>GGCUCGGCGGCGGA[2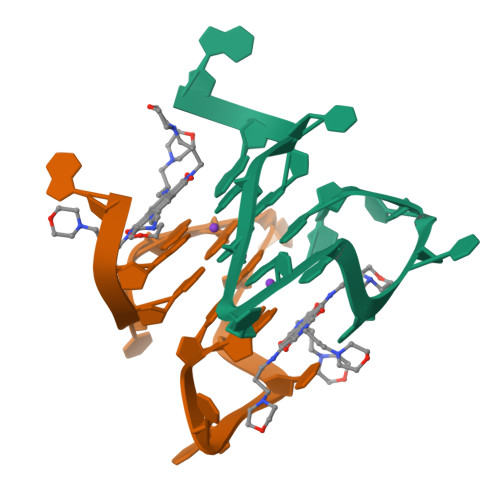x]> GMSIVLICNGGHEYYECGGACDNV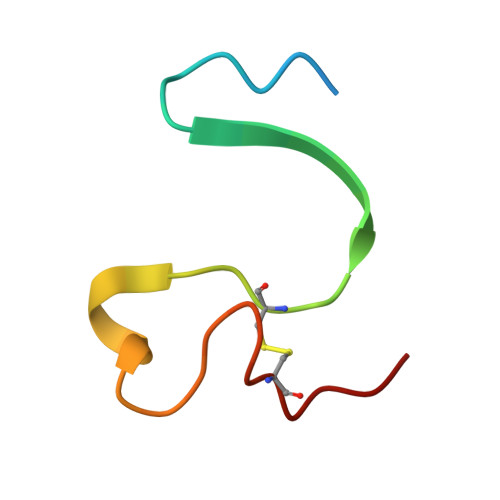CADLHIQNKTNCPIIN>[2x]GPMETTNWIGDENLTGNAEAPAKDDVVPDKNQFRYQKEELAAFCHFGPNTFNEIEWGE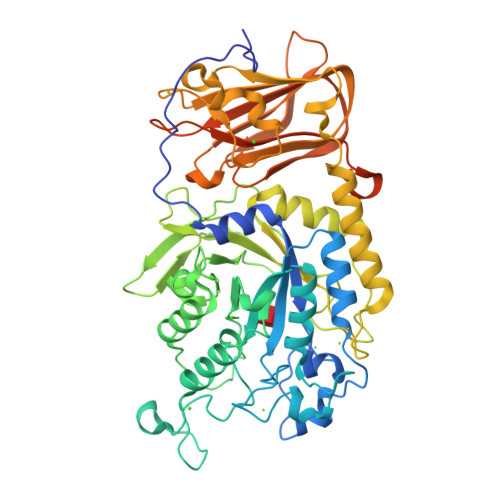HYGNQKPSEIFTLKNDFDAETLVKTLKDAGFKKLIVTAKHHDGFCIWDSEHTEYDVKASGYKNKNGESDILAEISKACTDQNMDMGLYLSPWDIHEPSYGYKDEHGNPTTPDKDAKDYNEFYNNQLEEILGNPKYGNDGHFVEVWMAGAKGSGANAQEYDFKKWFKTIQDNEGKAAGYDADCMLFGAEAYTTVRWIGNELGIAGKDTWSKSKVDKDKNTINSNKQGNATVGFEDGDQWTVPEADARITSGWFWGTKKNTPKTMEELSDMYFNSVGHNATLLLNVPPNNQGTVDKAILDRVTEFGNNIKATFKTNLAKAEGASVKVSEVRGGAKEYKPGNMIDDNDETYWATSDGKKSGEILIDLGKETKFDVVSIEEAIQNGQRINNYKVEYRNGDSGTWTLLEEGKTIGAKRLCRTSETTARQIKITVGTCDGKVPMISEIGVYKSTEDMEKPNPIPKGMEVIDVEDKDVADGKGFTFKGKWNPENQPQYING>GSHMQDPLSGLTDQERTLLGLLSEGLTNKQIADRMFLAEKTVKNY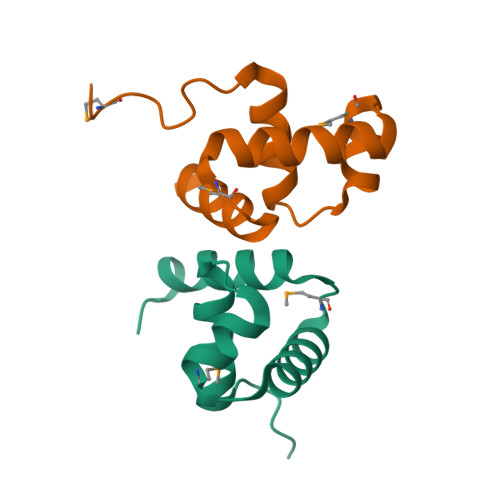VSRLLAKLGMERRTQAAVFATELKRSRPPGDGP[8x]>MMITLRKLPLAVAVAAGVMSAQAMAMACAGGGSTPLPLPQQQPPQQEPPPPPVPLASRAACEALKDGNGDMVWPNAATVVEVAAWRDAAPATASAAALPEHCEVSGAIAKRTGIDGYPYEIKFRLRMPAEWNGRFFMEGGSGTNGSLSAATGSIGGGQIASALSRNFATIATDGGHDNAVNDNPDALGTVAFGLDPQARLDMGYNSYDQVTQAGKAAVARFYGRAADKSYFIGCSEGGREGMMLSQRFPSHYDGIVAGAPGYQLPKAGISGAWTTQSLAPAAVGLDAQGVPLINKSFSDADLHLLSQAILGTCDALDGLADGIVDNYRACQAAFDPATAANPANGQALQCVGAKTADCLSPVQVTAIKRAMAGPVNSAGTPLYNRWAWDAGMSGLSGTTYNQGWRSWWLGSFNSSANNAQRVSGFSARSWLVDFATPPEPMPMTQVAARMMKFDFDIDPLKIWATSGQFTQSSMDWHGATSTDLAAFRDRGGKMILYHGMSDAAFSALDTADYYERLGAAMPGAAGFARLFLVPGMNH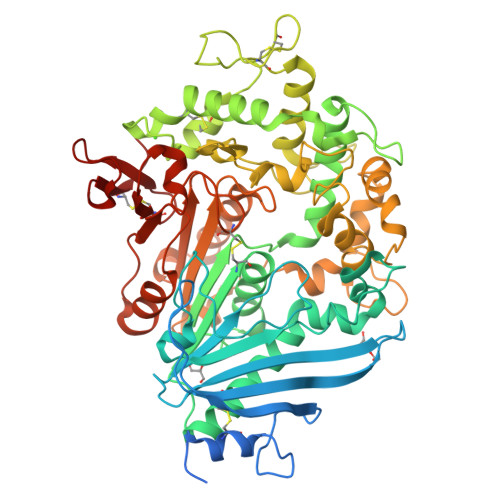CSGGPGTDRFDMLTPLVAWVERGEAPDQISAWSGTPGYFGVAARTRPLCPYPQIARYKGSGDINTEANFACAAPP[3x]> MAKEWGYASHNGPDHWHELFPNAKGENQSPIELHTKDIRHDPSLQPWSVSYDGGSAKTILNNGKTCRVVFDDTYDRSMLRGGPLPGPYRLRQFHLHWGSSDDHGSEHTVDGVKYAAELHLVHWNPKYNTFKEALKQRDGIAVIGIFLKIGHENGEFQIFLDALDKIKTKGKEAPFTKFDPSSLFPASR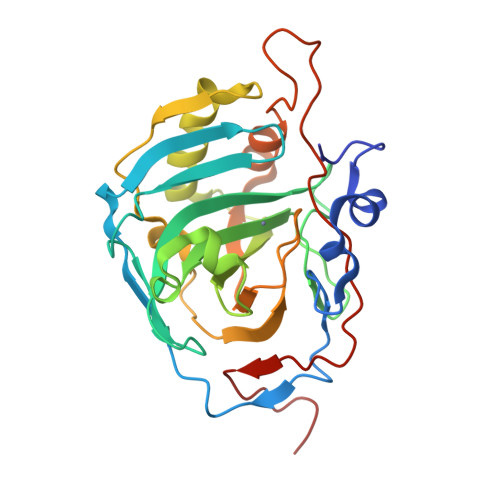DYWTYQGSLTTPPCEECIVWLLLKEPMTVSSDQMAKLRSLLSSAENEPPVPLVSNWRPPQPINNRVVRASFKHHHHHH HYDROXY(1-NAPHTHYL)METHYLPHOSPHONIC ACID | C11 H11 O4 P 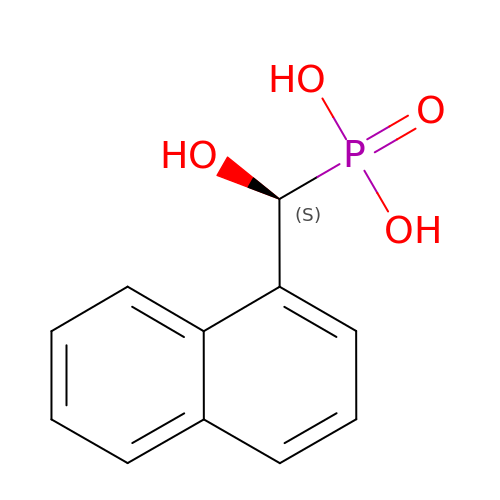| AXIBZLYWMBUYRV-NSHDSACASA-N> GLTGHGSSVLEELVQLVAAANIDISIKYDPRKDSEVFANRVITDDIELLKKILAYFLPEDAILKGGHYDNQLQNGIKRVKEFLESSPNTQWELRAFMAVMHFSLTADRIDDDILKVIVDSMNHHGDARSKLREELAELTAELKIYSVIQAEINKHLSSSGTINIHDKSINLMDKNLYGYTDEE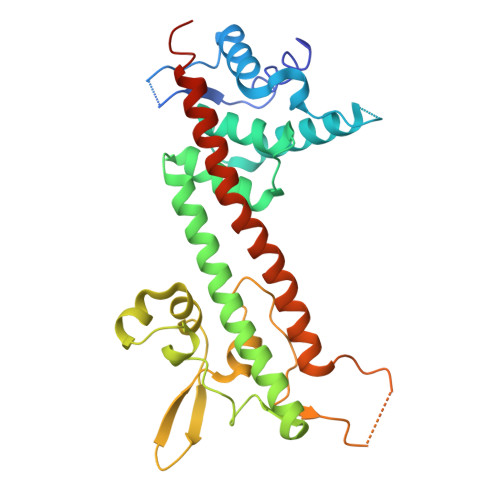IFKASAEYKILEKMPQTTIQVDGSEKKIVSIKDFLGSENKRTGALGNLKNSYSYNKDNNELSHFATTCSDKSRPLNDLVSQKTTQLSDITSRFNSAIEALNRFIQKYDSVMQRLLDDTSGKHHHHHH>[2x]MAKRVNTCKCVATPQEKIEYKTKVSRNSNMSKLQAGYLFPEIARRRSAHLLKYPDAQVISLGIGDTTEPIPEVITSAMAKKAHELSTIEGYSGYGAEQGAKPLRAAIAKTFYGGLGIGDDDVFVSDGAKCDISRLQVMFGSNVTIAVQDPSY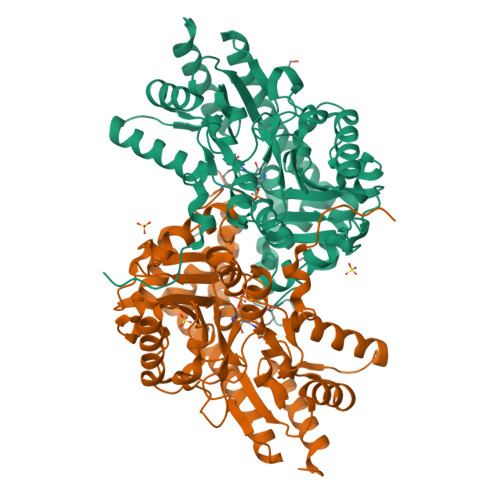PAYVDSSVIMGQTGQFNTDVQKYGNIEYMRCTPENGFFPDLSTVGRTDIIFFCSPNNPTGAAATREQLTQLVEFAKKNGSIIVYDSAYAMYMSDDNPRSIFEIPGAEEVAMETASFSKYAGFTGVRLGWTVIPKKLLYSDGFPVAKDFNRIICTCFNGASNISQAGALACLTPEGLEAMHKVIGFYKENTNIIIDTFTSLGYDVYGGKNAPYVWVHFPNQSSWDVFAEILEKTHVVTTPGSGFGPGGEGFVRVSAFGHRENILEACRRFKQLYKHHHHHH>[2x]METLRVSSKSRPNSV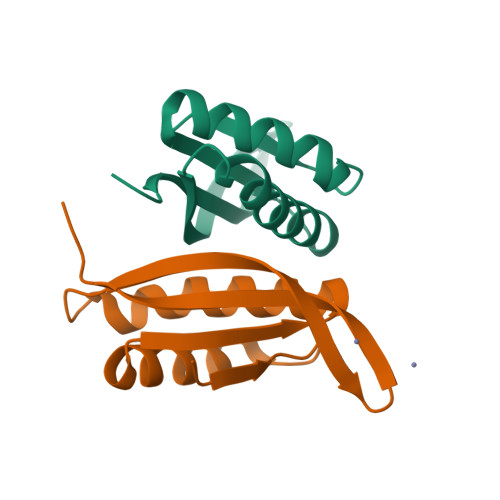AGAIAAMLRTKGEVEVQAIGPQAVNQAVKAIAIARGYIAPDNLDLVVKPAFVKLELENEERTALKFSIKAHPLET>MKIFLDTANIDEIRTGVNWGIVDGVTTNPTLISKEAVNGKKYGDIIREILKIVDGPVSVEVVSTKYEGMVEEARKIHGLGDNAVVKIPMTEDGLRAIKTLSSEHINTNCTLVFNPIQALLAAKAGVTYVSPFVGRLDDIGEDGMQIIDMIRTIFNNYIIKTQILVASIRNPIHVLRSAVIGADVVT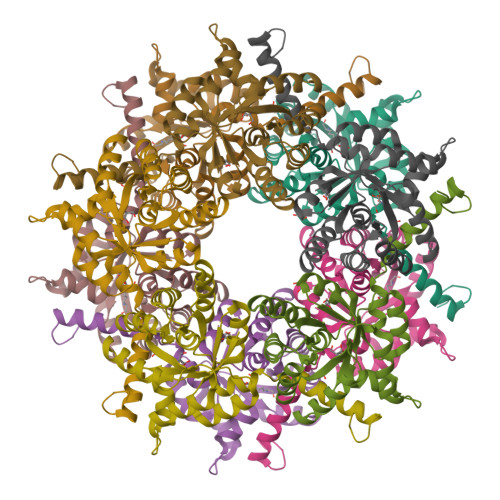VPFNVLKSLMKHPKTDEGLAKFLEDWKKVSPDGKLIL[5x]>NSAMDWQKITEKMCDFIQEKVKNSQSQGVVLGLSGGIDSALVATLCKRALKENVFALLMPTQISNKANLEDALRLCADLNLEYKIIEIQSILDAFIKQSENTTLVSLGNFAARIRMSLLYDYSALKNSLVIGTSNKSELLLGYGTIYGDLACAFNPIGSLYKSEIYALAKYLNLHENFIKKAPSADLWENQSDEADLGFSYTKIDEGLKALETNDEKLLRTLDPSLIAMLKNRMQKNAFKGKM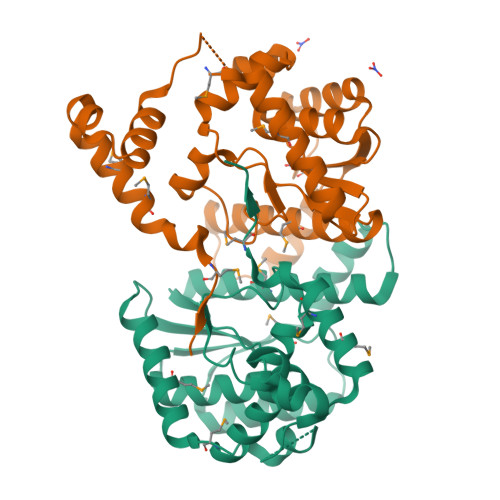PEILEI[2x]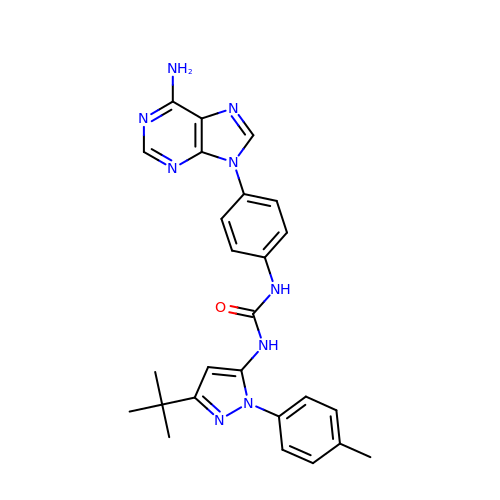1-[4-(6-amino-9H-purin-9-yl)phenyl]-3-[3-tert-butyl-1-(4-methylphenyl)-1H-pyrazol-5-yl]urea | C26 H27 N9 O | INQBVHWEOAKYED-UHFFFAOYSA-N>MAEAEAGGDEARCVRLSAERAKLLLAEVDTLLFNCDGVLWRGETAVPGAPETLRALRARGKRLGFITNNSSKTRTAYAEKLRRLGFGGPVGPEAGLEVFGTAYCSALYLRQRLAGVPDPKAYVLGSPALAAELEAVGVTSVGVGPDVLHGDGPSDWLAVPLEPDVRAVVVGFDPHFSYMKLTKAVRYLQQPDCLLVGTNMDNRLPLENGRFIAGTGCLVRAVEMAAQRQADIIGKPSRFIFDCVSQEYGINPERTV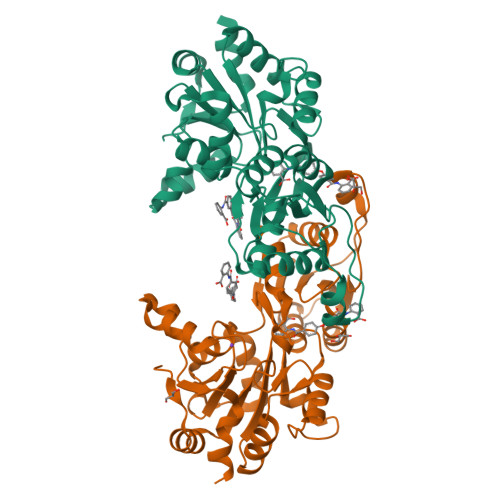MVGDRLDTDILLGSTCSLKTILTLTGVSSLEDVKSNQESDSMFKKKMVPDFYVDSIADLLPALQG[2x]>SLHSPGKAFRAALTKENPLQIVGTINANHALLAQRAGYQAIYLSGGGVAAGSLGLPDLGISTLDDVLTDIRRITDVCSLPLLVDADIGFGSSAFNVARTVKSMIKAGAAGLHIEDQVGAKRSGHRPNKAIVSKEEMVDRIRAAVDAKTDPDFVIMARTDALAVEGLDAAIERAQAYVEAGAEMLFPEAITELAMYRQFADAVQVPILANITEFGATPLFTTDELRSAHVAMALYPLSAFRAMNRAAEHVYNVL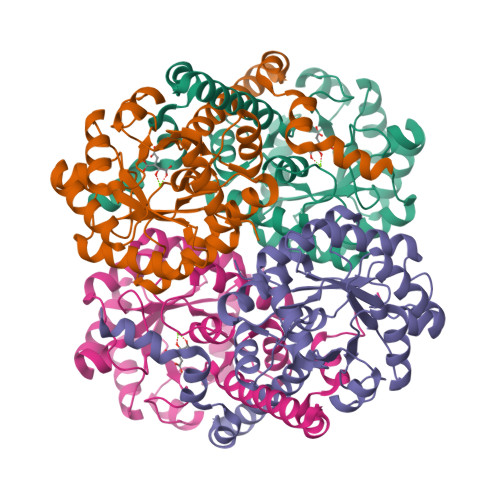RQEGTQKSVIDTMQTRNELYESINYYQYEEKLDNLFARSQVK[4x]> GPRNLRVLLDTAIPPSFCDTVSSVLLDDFNMVSLIRTSPADSLATIKQDNAEIDIAITIDEELKISRFNQCVLGYTKAFVVAHPQHPLCNASLHSIASLANYRQISLGSRSGQHSNLLRPVSDKVLFVENFDDMLRLVEAGVGWGIAPHYFVEERLRNGTLAVLSELYEPGGIDTKVYCYYNTALESERSFLRFLESARQRLRELGRQRFDDAPAWQPSIVETAQRRSG

A promising target for QS inhibitors (QSI) in PA is Pseudomonas quinolone signaling receptor (PqsR), also called multiple virulence factor regulator (MvfR). PqsR is a transcriptional regulator that controls the Pseudomonas quinolone signaling (PQS) system and is considered as one of the master regulators of PA virulence. Activation of PqsR by its native agonist PQS leads to the direct and indirect transcriptional modulation of genes responsible for environmental adaptation, virulence factor expression, iron acquisition, redox signaling, antibiotic tolerance, cytotoxicity, and immune modulation/evasion. Herein, this work reports the rational design, optimization, and in‐depth profiling of a new class of Pseudomonas quinolone signaling receptor (PqsR) inverse agonists.

However, compound 24 was chosen as our frontrunner as it showed the best compromise in the biological activities together with suitable solubility. We solved the crystal structure of 24 in complex with PqsR at a resolution of 2.74 Å. Overall, the observed binding mode was in accordance with previously reported QSI bearing the trifluoromethylpyridine headgroup. Notably, the detected electron density confirmed a more planar conformation of the bi‐aryl ring system in 24. Upon binding to PqsR, both rings tilted about 24° as observed by the corresponding dihedral angle. In comparison to the values shown in Figure 2, this would translate to an angle of 156° between both ring systems, which is closer to 180° (full planarity) than 119°. Investigating the complex more closely revealed that the meta‐chloro substituent of the Eastern ring fills a small pocket near Ile186, while the isopropoxy group protrudes into a tunnel‐like cavity framed by Ile186 and Tyr258. We conclude that the planar conformation promotes this space‐filling mode‐of‐interaction, rendering the pyrimidine scaffold beneficial for achieving high affinity. The binding mode to PqsR was elucidated by an X‐ray cocrystal structure.> 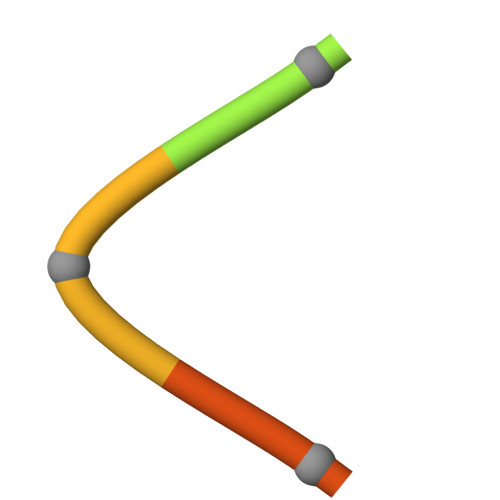FSHPQNT>SPDKLKKVLDKLRLKRKDISEAAETVNKVVERLLRRMQKRESEFKGVEQLNTGSYYEHVKISAPNEFDVMFKLEVPRIELQEYYETGAFYLVKFKRIPRGNPLSHFLEGEVLSATKMLSKFRKIIKEEVKEIKDIDVSVEKEKPGSPAVTLLIRNPEEISVDIILALESKGSWPISTKEGLPIQGWLGTKVRTNLRREPFYLVPKNAKDGNSFQGETWRLSFSHTEKYILNNHGIEKTCCESSGAKCCRKECLKLMKYLLEQLKKEFQELDAFCSYHVKTAIFHMWTQ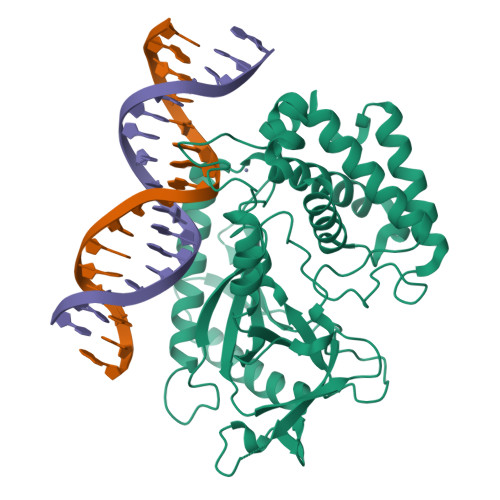DPQDSQWDPRNLSSCFDKLLAFFLECLRTEKLDHYFIPKFNLFSQELIDRKSKEFLSKKIEYERNNGFPIFDKL[2x]> MILLAVLFLCFISSYSASVKGHTTGLSLNNDRLYKLTYSTEVLLDRGKGKLQDSVGYRISSNVDVALLWRNPDGDDDQLIQITMKDVNVENVNQQRGEKSIFKGKSPSKIMGKENLEALQRPTLLHLIHGKVKEFYSYQNEAVAIENIKRGLASLFQTQLSSGTTNEVDISGNCKVTYQAHQDKVIKIKALDSCKIARSGFTTPNQVLGVSSKATSVTTYKIEDSFVIAVLAEETHNFGLNFLQTIKGKIVSKQKLELKTTEAGPRLMSGKQAAAIIKAVDSKYTAIPIVGQVFQSHCKGCPSLSELWRSTRKYLQPDNLSKAEAVRNFLAFIQHLRTAKKEEILQILKMENKEVLPQLVDAVTSAQTSDSLEAILDFLDFKSDSSIILQERFLYACGFASHPNEELLRALISKFKGSIGSSDIRETVMIITGTLVRKLCQNEGCKLKAVVEAKKLILGGLEKAEKKEDT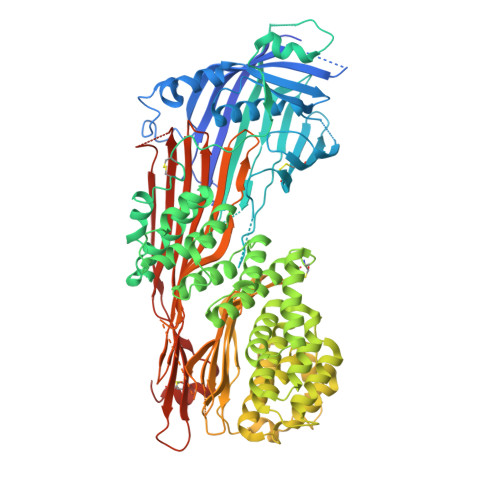RMYLLALKNALLPEGIPSLLKYAEAGEGPISHLATTALQRYDLPFITDEVKKTLNRIYHQNRKVHEKTVRTAAAAIILNNNPSYMDVKNILLSIGELPQEMNKYMLAIVQDILRFEMPASKIVRRVLKEMVAHNYDRFSRSGSSSAYTGYIERSPRSASTYSLDILYSGSGILRRSNLNIFQYIGKAGLHGSQVVIEAQGLEALIAATPDEGEENLDSYAGMSAILFDVQLRPVTFFNGYSDLMSKMLSASGDPISVVKGLILLIDHSQELQLQSGLKANIEVQGGLAIDISGAMEFSLWYRESKTRVKNRVTVVITTDITVDSSFVKAGLETSTETEAGLEFISTVQFSQYPFLVCMQMDKDEAPFRQFEKKYERLSTGRGYVSQKRKESVLAGCEFPLHQENSEMCKVVFAPQPDSTSSGWF> MGSHHHHHHSERTVRKNQATLTADEKRRFVDALVALKRSGRYDEFVTTHNAFIMGDTDSGERTGHRSPSFLPWHRRFLIEFEQALQAVDPSVALPYWDWSTDRTARASLWAPDFLGGSGRSLDGRVMDGPFAASTGNWPVNVRVDSRTYLRRTLGGGGRELPTRAEVDSVLAMSTYDMAPWNSASDGFRNHLEGWRGVNLHNRVHVWVGGQMATGVSPNDPVFWLHHAYIDRLWAQWQSRHPGSGYVPTGGTPNVVDLNETMKPWNDVRPADLL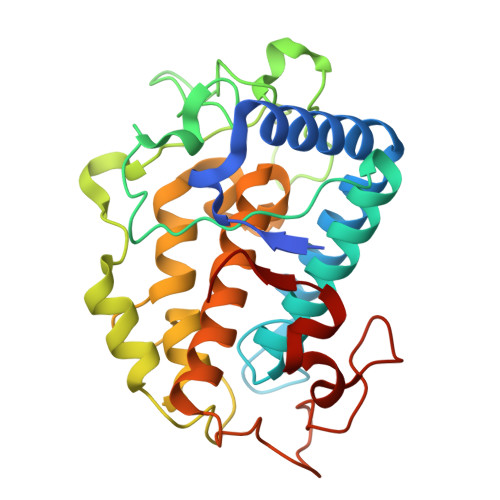DHTAHYTFDTV> CGACG;> GCCGC;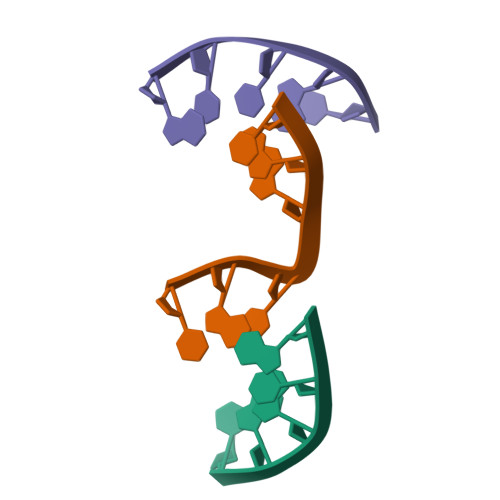> CGTGGC> SMNTPREVTLHFLRTAGHPLTRWALQRQPPSPKQLEEEFLKIPSNFVSPEDLDIPGHASKDRYKTILPNPQSRVCLGRAQSQEDGDYINANYIRGYDGKEKVYIATQGPMPNTVSDFWEMVWQEEVSLIVMLTQLREGKEKCVHYWPTEEETYGPFQIRIQD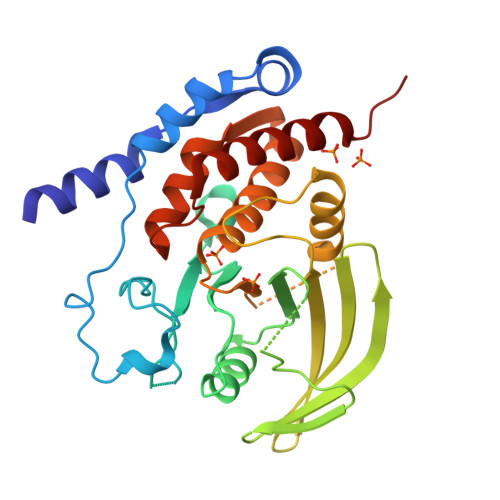MKECPEYTVRQLTIQYQEERRSVKHILFSAWPDHQTPESAGPLLRLVAEVEESPETAAHPGPIVVHCSAGIGRTGCFIATRIGCQQLKARGEVDILGIVCQLRLDRGGMIQTAEQYQFLHHTLALYAGQLPEEP> 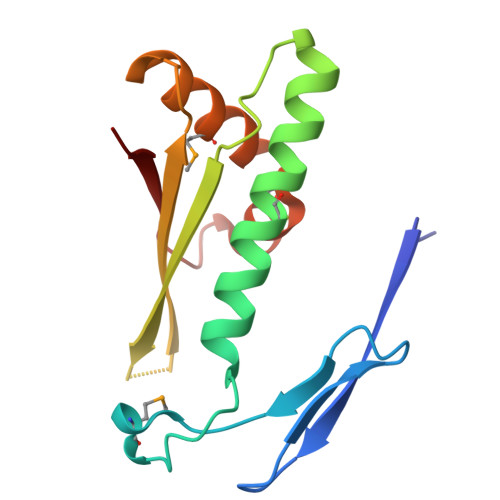MANVYTAEATATGGRAGTTRSSDDRLNLDLSVPAEMGGDGGPGTNPEQLFAAGYAACFQGALGVVSRRNKIDVPADSTITARVGLQKAGLAFALDVELEGHFPGLSREQAEGLMHAAHEVCPYSAATRNNVDVRLKVRE>MNSGLSRLGIALLAAMFAPALLAADLEKLDVAALPGDRVELKLQFDEPVAAPRGYTIEQPARIALDLPGVQNKLGTKNRELSVGNTRSVTVVEAKDRTRLIINLTALSSYTTRVEGNNLFVVVGNSPHHHHHHHHAGASVASAAPVKASPAPASYAQPIKPKPYVPAGRAIRNIDFQRGEKGEGNVVIDLSDPTLSPDIQEQGGKIRLDFAKTQLPDALRVRLDVKDFATPVQFVNASAQSDRTSITIEPSGLYDYLVYQTDNRLTVSIKPMTTEDAERRKKDNFAYTGEKLSLNFQDIDVRSVLQLIADFTDLNLVASDTVQGNITLRLQNVPWDQALDLVLKTKGLDKRKLGNVLLVAPADEIAARERQELEAQKQIAELAPLRRELIQVNYAKAADIAKLFQSVTSDGGQEGKEGGRGSITVDDRTNSIIAYQPQERLDELRRIVSQLDIPVRQVMIEARIVEANVGYDKSLGVRWGGAYHKGNWSGYGKDGNIGIKDEDGMNCGPIAGSCTFPTTGTSKSPSPFVDLGAKDATSGIGIGFITDNIILDLQLSAMEKTGNGEIVSQPKVVTSDKETAKILKGSEVPYQEASSSGATSTSFKEAALSLEVTPQITPDNRIIVEVKVTKDAPDYQNMLNGVPPINKNEVNAKILVNDGETIVIGGVFSNEQSKSVEKVPFLGELPYLGRLFRRDTVTDRKNELLVFLTPRIMNNQAIAIGRGHHHHHHHH[14x];>MRKSLVALLLLAASG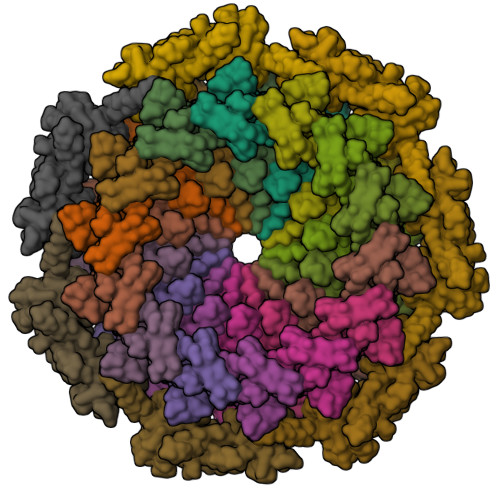LAQAQVDLREGHPDRYTVVRGDTLWDISGKFLRQPWKWPELWHANPQIQNPHLIYPGDTLSLVYVDGQPRLVLNRGESRGTIKLSPKIRSTPIAEAIPTIPLDKINSFLLANRIVDDEKTFTSAPYIVAGNAERIVSGTGDRIYARGKFADGQPAYGIFRQGKVYIDPKTKEVLGINADDIGGGEVVATEGDVATLALTRTTQEVRLGDRLFPTEERAVNSTFMPGEPSREVKGEIIDVPRGVTQIGQFDVVTLNRGQRDGLAEGNVLAIYKVGETVRDRVTGESVKIPDERAGLLMVFRTYKKLSYALVLMASRPLSVTDRVQNP[7x]>[8x]MTQPMPGKPAEDAENELDIRGLFRTLWAGKLWIIGMGLAFALIALAYTFFARQEWSSTAITDRPTVNMLGGYYSQQQFLRNLDVRSNMASADQPSVMDEAYKEFVMQLASWDTRREFWLQTDYYKQRMVGNSKADAALLDEMINNIQFIPGDFTRAVNDSVKLIAETAPDANNLLRQYVAFASQRAASHLNDELKGAWAARTIQMKAQVKRQEEVAKAIYDRRMNSIEQALKIAEQHNISRSATDVPAEELPDSEMFLLGRPMLQAELENLQAVGPAFDLDYDQNRAMLNTLNVGPTLDPRFQTYRYLRTPEEPVKRDSPRRAFLMIMWGIVGGLIGAGVALTRRCSKEFRVPGSHHHHHHHH

Lipopolysaccharides such as the enterobacterial common antigen are important components of the enterobacterial cell envelope that act as a protective barrier against the environment and are often polymerized by the inner membrane bound Wzy-dependent pathway. By employing cryo-electron microscopy we show that WzzE, the co-polymerase component of this pathway that is responsible for the length modulation of the enterobacterial common antigen, is octameric with alternating up-down conformations of its L4 loops. The alternating up-down nature of these essential loops, located at the top of the periplasmic bell, are modulated by clashing helical faces between adjacent protomers that flank the L4 loops around the octameric periplasmic bell. This alternating arrangement and a highly negatively charged binding face create a dynamic environment in which the polysaccharide chain is extended, and suggest a ratchet-type mechanism for polysaccharide elongation.

The ConSurf analysis also revealed an arginine within α7 (R267) that interacts with the downward facing L4 to be highly conserved. To investigate how robust the alternating conformation of the L4 loops is, we replaced this residue with an alanine and a glutamic acid in two constructs. Although the change of this amino acid is clearly visible in the cryo-EM density map, replacement had little effect on the overall octameric structure of WzzE or the alternating arrangement of the L4 loops. Although there are only small differences between the native WzzE and both R267 variants, these variants do underscore the nature of the alternating loops in WzzE, as both structures of the mutants were solved independently using reference-free ab-initio starting volumes and clearly display the same pattern of alternating L4 loops in their unsymmetrized C1 maps as the native WzzE.> GSMDYKDDDDKKTNWLKRIYRVRPCVKCKVAPRNWKVKNKHLRIYNMCKTCFNNSIDIGDDTYHGHDDWLMYADSKEISNT

DNA sequencing of the output from this selection revealed a distant clone (clone 18-19) that differed from the consensus sequence at 15 out of 80 positions and bound ATP with far greater affinity and specificity than all other clones from that round of selection. The X-ray crystal structure for protein 18-19 was originally solved by Lo Surdo et al. and found to adopt a novel zinc-nucleated α/β-fold not yet observed by nature. The fold is characterized by an α-helix (residues 6–20), followed by an extended loop, then two short β-strands (residues 33–36 and 39–43), followed by a second α-helix (residues 46–56) that leads to another extended loop which terminates in a third β-strand (residues 64–68). A zinc metal ion is bound by tetrahedral coordination to four invariant cysteine residues at positions 23, 26, 46, and 49.

Protein 18-19 was the highest affinity clone isolated from round 18. Unlike many naturally occurring proteins, protein 18-19 requires high concentrations of free ligand in order to remain stably folded and soluble. We determined the X-ray crystal structures of protein 18-19 and the evolutionarily optimized variant, protein DX, to resolution limits of 2.8 Å and 1.65 Å, respectively. The structure of protein 18-19 was solved from the anomalous X-ray scattering of a zinc ion bound to the protein using multiwavelength anomalous dispersion (MAD) methods. The Cα backbone trace of proteins 18-19 and DX can be superimposed with a root mean square deviation (r.m.s.d.) of 0.51 Å from residues 7 to 71. In protein 18-19, Asp65 is located on the hydrophobic face of the third strand and forms a salt bridge with Arg21, while Asn32 is located on the polar face of the first strand and contacts the purine base of ATP through a bridging water interaction. Experiments performed in the absence of ATP showed that protein 18-19 forms an insoluble precipitate after 3 days, while proteins containing one or both of the selected mutations remain soluble after 7 days. Small differences in the relative positioning of the ATP molecules in the two protein structures cannot be resolved due to the limiting resolution of the 18-19 structure.>[2x]SNAMDRVATARAYYRALDEHDYDL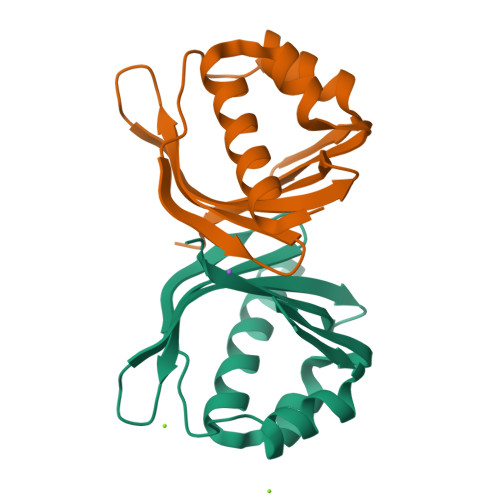LSDVLAPDFVHDRPDRTIEGRERFVRFMREERPQTDTSHPIATIYTGASTVAVEGRLLNSDGAEITQFVDVFAFEDGVIGRIRTHTPEP>[4x]GHPETLVKVKDAEDQLGARVGYIELDLNSGKILESFRPEERFPMMSTFKVLLCGAVLSRVDAGQEQLGRRI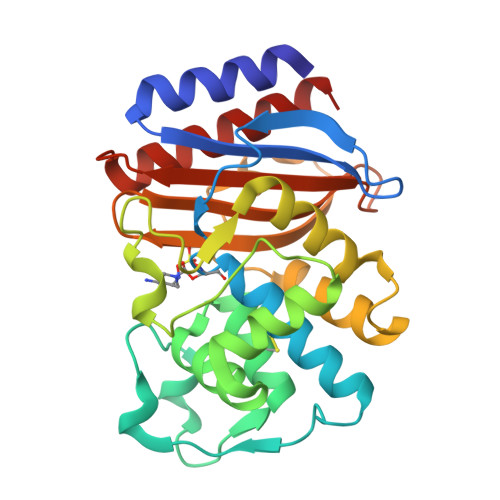HYSQNDLVEYSPVTEKHLTDGMTVRELCSAAITMSDNTAANLLLTTIGGPKELTAFLHNMGDHVTRLDRWEPELNEAIPNDERDTTTPAAMATTLRKLLTGELLTLASRQQLIDWMEADKVAGPLLRSALPAGWFIADKSGYGERGSRGIIAALGPDGKPSRIVVIYTTGSQATMDERNRQIAEIGASLIKHW> MLSRAIFRNPVINRTLLRARPGAYHATRLTKNTFIQSRKYSDAHDEETFEEFTARYEKEFDEAYDLFEVQRVLNNCFSYDLVPAPAVIEKALRAAR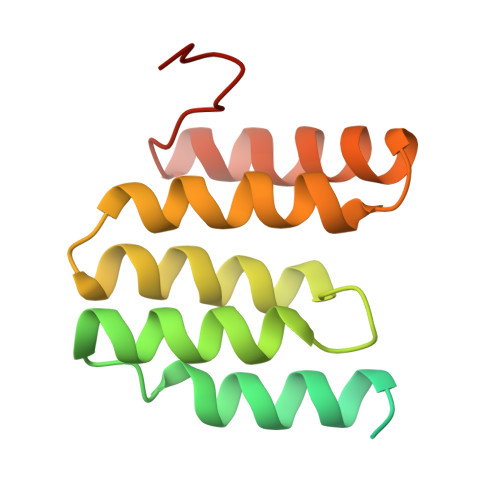RVNDLPTAIRVFEALKYKVENEDQYKAYLDELKDVRQELGVPLKEELFPSSS> GDRVKKLINSQISLLIGKGLHEFDSLRDPEVNDFRTKMRQFCEEAAAHRQQLGWVEWLQYSFPLQLEPSARGWRAGLLRVSNRALLVNVKFEGSEESFTFQVSTKDMPLALMACALRKKATVFRQPLVEQPEEYALQVNGRHEYLYGNYPLCHFQYICSCLHSGLTPHLTMVHSSSILAMRDEQSNPAPQVQKPRAKPPPIPAKKPSSVSLWSLEQPFSIELIEGRKVNADERMKLVVQAGLFHGNEMLCKTVSSSEVNVCSEPVWKQRLEFDISVCDLPRMARLCFALYAVVEKAKKARSTKKKSKKADCPIAWANLMLFDYKDQLKTGERCLYMWPSVPDEKGELLNPAGTVRGNPNTESA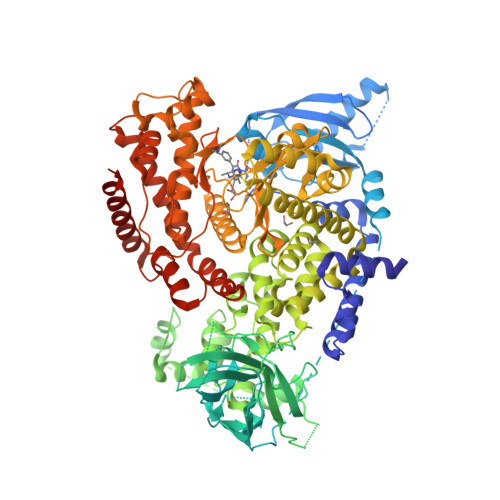AALVIYLPEVAPHPVYFPALEKILELGRIGERGRITEEELREILERRGSGELYEHEKDLVWKMRHEVQEHFPEALARLLLVTKWNKHEDVAQMLYLLCSWPELPVLSALELLDFSFPDCYVGSFAIKSLRKLTDDELFQYLLQLVQVLKYESYLDCELTKFLLGRALANRKIGHFLFWHLRSEMHVPSVALRFGLIMEAYCRGSTHHMKVLMKQGEALSKLKALNDFVKVSSQKTTKPQTKEMMHMCMRQETYMEALSHLQSPLDPSTLLEEVCVEQCTFMDSKMKPLWIMYSSEEAGSAGNVGIIFKNGDDLRQDMLTLQMIQLMDVLWKQEGLDLRMTPYGCLPTGDRTGLIEVVLHSDTIANIQLNKSNMAATAAFNKDALLNWLKSKNPGEALDRAIEEFTLSCAGYCVATYVLGIGDRHSDNIMIRESGQLFHIDFGHFLGNFKTKFGINRERVPFILTYDFVHVIQQGKTNNSEKFERFRGYCERAYTILRRHGLLFLHLFALMRAAGLPELSCSKDIQYLKDSLALGKTEEEALKHFRVKFNEALRESWKTKVNWLAHNVSKDNRQ>[2x]MVQLEPNITLVLKHLASCGAVVSAEQQAALDHSIPIKRIEAGLRSLTLWGRLTTLNGKDYLVAEGYNVASSKEGAAVYETKYFYSQDGARWSDLQPVDSETATRCARIKGMLSGDPAKNYELEEKDPNAPEPSPEAEEEVKPLVFQIPELAVLRCRVDAIATATSVIPTDSTILNAASQVVPNRLFAGAAYPEKLESYQHRFSLPGSGVTLSQDLRGTWAVQYDAFKGVAQVRSLLFPGYFFYYAANELTWGSLYVGDGLRNNDLIFML;> GMAAVDSVAQALAYLQVHSPQDGTSMYDHLVKLVSKVLEDQPKNAVDLLETSLLVKKSTFDPKESSPLVPIPVAPDATQTQAAVSIFGDPELPINPATGEPVPADPPNEFEAENMLGAAAVLDCLGVGLGRELGVNIALAAKRIGEDPKLAVRSVRFFGKFLGLYSDYFVFEVAFKKEAAKEAAPAAPAPERVEGEAASSSAPEVPVEEPGKGANKFTYLVCSSLGGPLTRLPDVTPAQVKASRRIKKLLTGRLTSHVSTYPAFPGNEANYLRALIARISAATVVAPSDLFSLNDETGELERAEDWEPPAGREMAAPTAWVHVRPHLKSQGRCEVHKRELPEDADEDEFYNEDELEEGPDLLAALEEDAQLPGEQAAWTPIYSSASEAVKTQAGGLRSLVWPGAVCGGRGSEWTCVYVGWGVKNAPFVPLPPPPVAQEFAWGEVETQELELKPAPPPPEEEAEADE;> MAADVGQALAFLQQVKTTQGASIYEGLKAALAKVLEDRPVNAVEALETSVLSTPPAANLSVPLVPAASAAAAAAAVAKASLFGDPEPVLDPESGEPIDPDAPNEFECEDVEGDGDLLDGLGVGLGRQEMYAAMLAVKRLGEDAKRGVSTVRFFGKFFGTQADYYVFETTLQSNPDMPEAPEGTIPLEPYGEGVNAYIYFVSNTLGGPLQQLPYVTPEQIKASRLLRRYLTGRLDAPVSAFPAFPGNEANYLRALIARISAATVCCPRGFFTADDDSAELSANDEWVPLKGREMALPVNWSHRYAHLKGQGRTVTHKRDPPDEEEEPEKNFWTAEEMEAGPPPLATLDTDAPLPAATGDKVPPPAWSPVFASASVTTRNQVAGVRSNRWPGAVCACAGRHFTSMYVGWGIKAGGEWSPCPPPPPVPQWGAPAAGVEGGQQLLLECNDLPPKPAPPEEEDE;> MADDELPPQPVWEGPLDEDGKPHGLGKMEYPPPPMGEDDEEEKPGDKFEGTMEHGVRTGKGTYTWGVSGAVYTGDYVNGKKHGKGKMVYPDKGVYEGDWVEDVMQGQGTYTYPNGDIYQGAFWAGKRHGKGMYHYKGPCCQLVGDWADGGFTYGRWVYADGSMFMGKFGGAAADSKPTAGSYFYSSSSLVQEGHFAKDGSWVGHRDPAVGKEFSVA;> MALGPFVLPFRGDQYSFGINFKSSPEEKLNFDLSCVAFDVKGQLHDTLHARKPTALDGALVKGFEKQALPEETVQVEGDDVIYMFPKKFERQVEVLLFVASAPSIPGKKHDLDSSSKLEFAVSYSDVGGQAFNQSFDLKPLAAQGGVSSIIVAVMYLQAEGGWTLRSVGDCHPFDSPGLIVPELKQTILNLRDHHGVQLDAADAIQAIDPAERVPVTRQFQDQSLDEASAGRAAEPAPVKKLRIDLSWTFWPPPPPTEEGEEPPEEPALEYNLVMYNKDGEEVQSISTGNREATGARAGRPEPEEDEEEEKEEEKEEPEEGEEGEEGEGGEPKEPPPPPPAPKVDPYEFKERDVIYLDVPDLPAEVRSMVLLVTNYDEENGFTRVRTVRCRLVDVSNGEAPLPGSKAAVAAAAAAAEQGLAAPPNPERVLADYGVLSKYEDDKATTQVALMKLYKEYADSAFNVFRGAGVDNVAAFIGQEPDTIINQLKAYLEATKKQKAAEAAAAAAAEESGEEITADPKPHVWRFRALGLNFGGDSLEAIEHDLKNLFAFDGDLAPGAARDSDTSRSSFPNGDTYFGSYADDVKHGPGLYAFATGAGYAGEYAGGKRHGRGVMVFPDGGTYVGEFVADKFEGQGQYRYPDGSVYTGSWAAGQKHGPGVYWDTARGCLRGEWKKGLLVGKGTYEQPALRFEGEFVRGMPAGTATYTLTGHRTLDMPCFAAQHIQAEEGPTLALPCAYGIPPGSGDEPQLDEEGQPIEDTDKPPLPAHPKYEGLTFTAEQLPGAAPDTVFPPEEGKPVPITAVPAFSVSTGLVA;> GAAAEPILEVLVGKVLEQGLMEVLEEEELAAMRAHQEHFEQIRNAELVATQRMEAAERRKLEEKERRMQQERERVERERVVRQKVAASAFARGYLSGIVNTVFDRLVSSGYIYDPVMREVETAFMPWLKEQAIGYLARGVVARRVVDKLVEDAAAALAANRSTLADKAASTAATVDAWAERQAKMEAELQGKELEAVRRRPTFVLRELKPAVASADAVEAAAAELTAQAEEAANAKWEADKAEAAEKARAEAEAAAEEQKALLEELAATAAAEAEERGEEPPAEPPSLPDGVEPVDVEAEVAKAVEAVPKPPVKEVTDIDILSYMMDKGAITKDAIIQALAVHALGDKAYTNHPAFAEAEGA;> MSEPGEEPVAAPAGPAPDPVLNELYGSERPAVELLPGVPLSPIVNSCWLPADAKAMLAESWIPVPPEDAGEEAGPPPPAFEAAAPEYNELVRRLAKTAPFRKWNELTIQAKQLEQEVAGLKGPDAEAKQAELENVKVQIADAEAAVAEVKQSFSDDPLSLTGWMQALTDLADGGMTTFEVSGQGWPYCSLRQLFGEMPSAAPPAGFFDGVERVLGTFKRRYEKERGPGSVQLMLKLAPNVFSDAWSTGGAPAAVAAVEAYVERARANVFGPDGGVTPEGVPEPLDLVQLVWWDFAAADPLPVLKALQRMATDQLQVDEDSGEVSVSEPKKIRGIGLVDFPADRLKAAIQAGVPITCVQVEHSVLVRSAQPVLDLCAKYGIKVLARGGTLGGLLSAKYLGAPPPDPVRGDADLDSVPGCLDAVNNVGGWARLQAALAVIKGIADKHGVKPETVALRWQIDAGCFPLVTTRWSSRVWRQFGYEGWSSFEVSGGRPGVDGPLFQVESFLDVEDVRALAGLAAVHLGPKAG;> MAPTQAGHDTAYLKETVGEALARGCAAAISAQPNDPVEYLGLWLLKYVKNAEVEGNFYRERQQDLQKKKDRLVKEAQSEQAAKSVALTRKEAADALALVTAEPRELLEAAVKLVKQHTAAGAAYAAVVAEPEEPDWVAPEDDEAAAVETEDEAAGGAALAEGEEPPPEPEPEPEAAPEDGEGDAPAPKIPRPVDYSKKYFAYVAASAGQEHVLEADLYRPAPPPEDADEDFKPEPLPYSFRVLDEKLPMLYVPNVAAEERVKFFRKFPKIGSYQACGVALPASGEFKALLAADTLFPEGSGQPLSADDRDFVWEVSQSLSRALEAVQARAAEALAATSAAEAVEELKAKVAELREQAAAEAAAAAPPPPAEGEEGEGEAPPAEEEPPAEEEAEEEEEEAEEGAEEGAEEGEEGEEAPPKPKKKKKVFNPIPGLQAAIEKLTAAAEAATEADARAQAAVALEKQALDEVVALASSHSDATLSSLRNMLSVPQGTYHVVKALLHLLGRPAASFSTWKRAHSHFSPRLFEDMAAYDATAERDMAVWGRVRS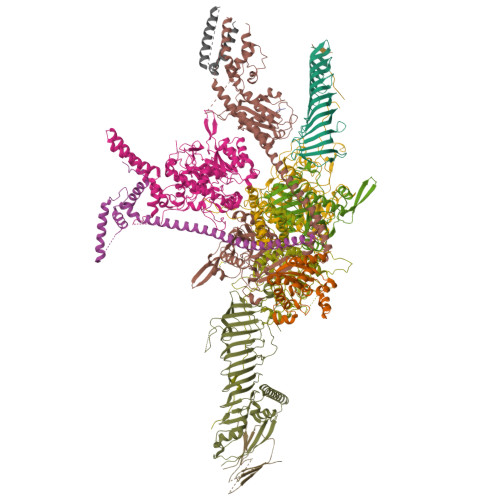CYKAAPAAKKLDAEMPNTLFGSVALMYIKQVRRVARKAVLQRELAAKLAKAQQDLADKQAALVEAERVKAEREAEEARLAAEAEAAAAAEAEAAARAAAEAEAAAAAEAAAEAAAEAAAAAAEAAAEAGEGEAVAEREAAPAEAEAAPAEGEAAPPAEGEGEAQPAQEGSNSSSSSSDSSSSEESKAAAE;> MAELEKTFALIKPDAVRAGKAQEIMQLIELNGFTIIAKQKLQLTRARAEEFYGEHKGKEFFPKLVNFMTSGPIWALVLAKPGAILAWRALMGPTNVFKARAEQPKCLRALYGTDGTQNATHGSDSPISAAREIKFFFPTLSGDPTIYAEPTAAAEYITKRIQPALAKALAALAREKPSADKFEAITFVAGYLLQNNPNKPKVLMPDEWDPALMGDDEDDEADFINARLAAPTGNDGATKAEFDAMVEAAKADTGGAAPAQEFVYPDSKPTTPVVPAPPAPGSKPPSASGARPQSARPTSARPPSASAAPPAPLAPVPPPASSSRPASGSGRPPSATARPPSATPPPPPPAVELEEADDPAQLDEAATKVQAAFRGYQARKEVAVMRSEAQPGEAAAEPEQEAELQPEAEPEPQPEGEQEPQPQASASSSFLPDGVTEEMAAEAATRVQAHMRGHLARKQVAAIKAQQAAPAVAESSEALAEPEPQPEAEAEPQPQASVSSSFLPDGVTEEMAAEAATLVQAHMRGHLARKQVAAIKAQQAAPAVAESSEAQAEAEQTEAEAEPQPDAEAEAGAAEGEAEPEPEAAE>MGSSHHHHHHQQKLTSPDNNLVMTFQVDSKGAPTYELT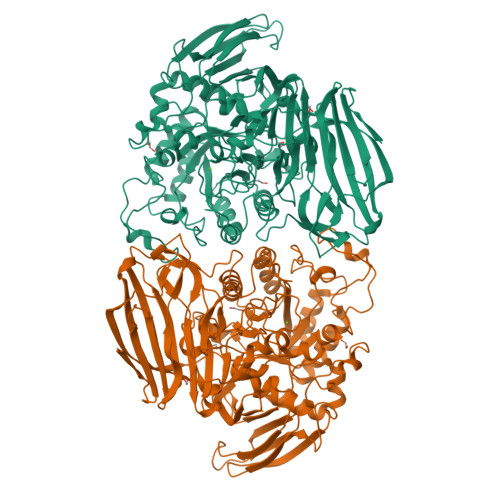YKNKVVIKPSTLGLELKKEDNTRTDFDWVDRRDLTKLDSKTNLYDGFEVKDTQTATFDETWQPVWGEEKEIRNHYNELAVTLYQPMNDRSIVIRFRLFNDGLGFRYEFPQQKSLNYFVIKEEHSQFGMNGDHIAFWIPGDYDTQEYDYTISRLSEIRGLMKEAITPNSSQTPFSQTGVQTALMMKTDDGLYINLHEAALVDYSCMHLNLDDKNMVFESWLTPDAKGDKGYMQTPCNTPWRTIIVSDDARNILASRITLNLNEPCKIADAASWVKPVKYIGVWWDMITGKGSWAYTDELTSVKLGETDYSKTKPNGKHSANTANVKRYIDFAAAHGFDAVLVEGWNEGWEDWFGNSKDYVFDFVTPYPDFDVKEIHRYAARKGIKMMMHHETSASVRNYERHMDKAYQFMADNGYNSVKSGYVGNIIPRGEHHYGQWMNNHYLYAVKKAADYKIMVNAHEATRPTGICRTYPNLIGNESARGTEYESFGGNKVYHTTILPFTRLVGGPMDYTPGIFETHCNKMNPANNSQVRSTIARQLALYVTMYSPLQMAADIPENYERFMDAFQFIKDVALDWDETNYLEAEPGEYITIARKAKDTDDWYVGCTAGENGHTSKLVFDFLTPGKQYIATVYADAKDADWKENPQAYTIKKGILTNKSKLNLHAANGGGYAISIKEVKDKSEAKGLKRL[2x]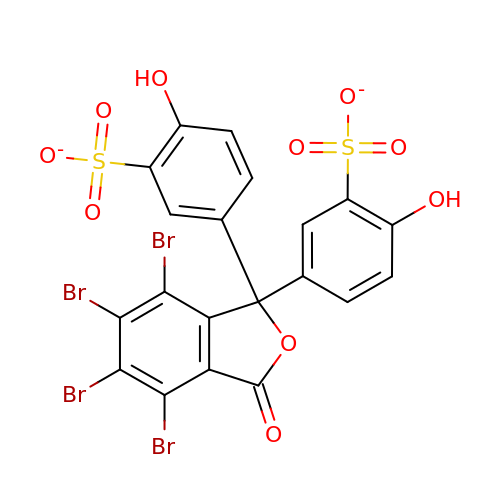3,3'-(4,5,6,7-TETRABROMO-3-OXO-1(3H)-ISOBENZOFURANYLIDENE)BIS [6-HYDROXYBENZENESULFONIC ACID]ANION | C20 H8 Br4 O10 S2 | OHTXTCNTQJFRIG-UHFFFAOYSA-L(1~{S},5~{S},6~{R})-10-[3,5-bis(chloranyl)phenyl]sulfonyl-5-(hydroxymethyl)-3-[(1~{S})-1-pyridin-2-ylethyl]-3,10-diazabicyclo[4.3.1]decan-2-one 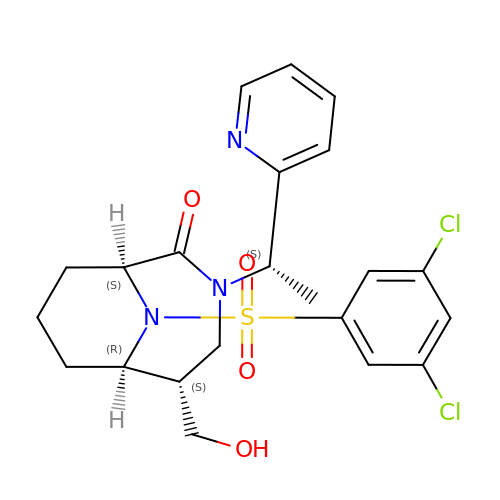| C22 H25 Cl2 N3 O4 S | UHJFWSJLAJJMIN-RSMHBEIYSA-N> MQQGQMAYSRAITVFSPDGRLFQVEYAREAVKKGSTALGMKFANGVLLISDKKVRSRLIEQNSIEKIQLIDDYVAAVTSGLVADARVLVDFARISAQQEKVTYGSLVNIENLVKRVADQMQQYTQYGGVRPYGVSLIFAGIDQIGPRLFDCDPAGTINEYKATAIGSGKDAVVSFLEREYKENLPEKEAVTLGIKALKSSLEEGEELKAPEIASIT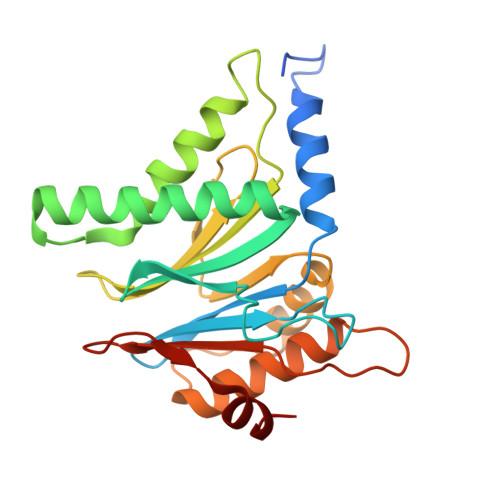VGNKYRIYDQEEVKKFL> FSSLRLSQKDARGSGYLPAQRFLSLLKASPEEYRSLLREATQAKIVDPAFLRVASQRFFALSDRFYPPEILDILSDFASFPYSDEALLAAVAGRLEDQLVEPSPKRLAALLSLSARLGLCHPSIRDPLTKHIEEKMYAFDAALLDSLCRTVGSLLSPRLPLLDGLATQAQLLASDLRAGEQSLETGDEVAQRRYIALLFRCLEGLSRQRYSQSALVDACVACAEQHGQAFPLHDTLRAVAAARRLDLAGIEEPLRRSDMADKVNRATDRGDQLLALLRHLDLLRLRDSQLLQKVSEAVELHSQK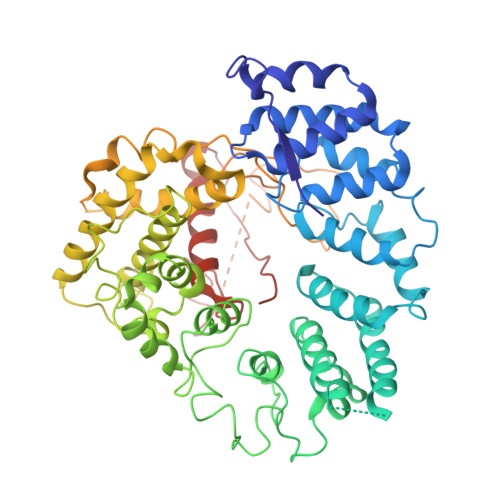AAFLATQLPEALLHLTRLAPADLRLPVALLSQPSLLAMAPRLSAAQLQQLLSASALVLFQHIQRREGGQGGDPLIAREAEALAKTVERFLDLLKPQFLSLNLRDRRALKEAASLFLVEAKGAAKSSAASPQFALAPKTVDFCCFLEEADVAPPLPLAPSGGVDFQSVGLVEACSRLVLCADARFSETRNSARGASEGDTKKGDSEKTSLPQTAGRDMEAAAKQRALLFVSPRDAFADARRSRGETVSKSSKAKEREETTTCKLGGVSTDLPVSITPQAASSLLLTQLALIRRGILRHEIQTCIPPP> SQEKVSIEQQLAVESIRKFLNSKTSYDVLPVSYRLIVLDTSLLVKKSLNVLLQNSIVSAPLWDSKTSRFAGLLTTTDFINVIQYYFSNPDKFELVDKLQLDGLKDIERALGVDQLDTASIHPSRPLFEACLKMLESRSGRIPLIDQDEETHREIVVSVLTQYRILKFVALNCRETHFLKIPIGDLNIITQDNMKSCQMTTPVIDVIQMLTQGRVSSVPIIDENGYLINVYEAYDVLGLIKGGIYNDLSLSVGEALMRRSDD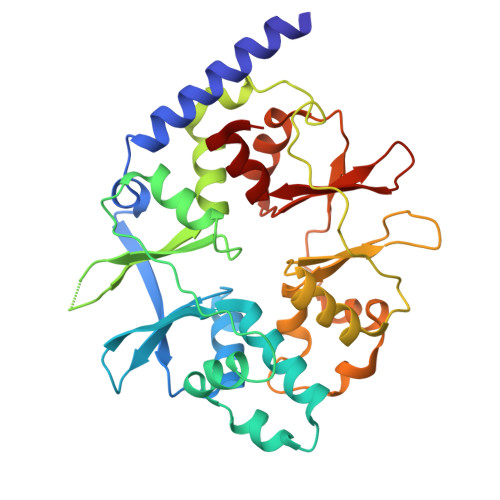FEGVYTCTKNDKLSTIMDNIRKARVHRFFVVDDVGRLVGVLTLSDILKYILLGS>[2x]GAMNAQAEEFKKYLETNGIKPKQFHKKELIFNQWDPQEYCIFLYDGITKLTSISENGTIMNLQYYKGAFVIMSGFIDTETSVGYYNLEVISEQATAYVIKINELKELLSKNLTHFFYVFQTLQKQVSYSLAKFNDFSINGKLGSICGQLLILTYVYGKETPDGIKITLDNLTMQELGYSSGIAHSSAVSRIISKLKQEKVIVYKNSCFYVQNLDYLKRYGPKLDEWFYLACPATWGKLN

The major regulator of virulence factors in L. monocytogenes is the transcription activator PrfA, a member of the Crp/Fnr family of regulators. PrfAWT is a homodimer in which each monomer consists of an N-terminal domain (residues 1 to 108) and a C-terminal DNA-binding domain (residues 138 to 237) linked by a long α-helix (αC, residues 109 to 137). Two α-helices in the C-terminal domain, αE (residues 170 to 178) and αF (residues 183 to 197), constitute the two helices of the typical HTH motif present in many prokaryotic transcription factors. Glutathione binding stabilizes the DNA-binding helix-turn-helix (HTH) motif in a conformation compatible with DNA-binding, thereby allowing expression of PrfA-regulated virulence factors.

In addition, we found three new PrfA mutants in the remaining three strains—Leu to His substitution at residue 140 (PrfAL140H), Ala to Gly substitution at residue 218 (PrfAA218G), and Ala to Val substitution at residue 94 (PrfAA94V). All the previously identified PrfA* mutants, i.e., PrfAG145S, PrfAG145C, and PrfAL140F, could grow in this medium with G-6-P, as could the PrfA mutants PrfAL140H and PrfAA218G, whereas the strain carrying the PrfAA94V mutation was unable to grow. The PrfAG145S, PrfAG145C, and PrfAL140F mutants showed the highest expression levels, followed by PrfAA218G and PrfAL140H. To gain a deeper understanding of the PrfA* mutant proteins, the crystal structures of purified PrfAL140H, PrfAL140F, and PrfAA218G were determined as individual proteins and in complex with the PrfA hly promoter DNA. We expected that the crystal structures of PrfAL140H, PrfAL140F, and PrfAA218G would be similar to the PrfAG145S structure, since our in vivo characterization classified them as PrfA* mutations. However, their structures showed that each of the PrfA* variants had only one folded HTH motif, with the remaining structure residing in the PrfAWT conformation. The PrfAL140H, PrfAL140F, and PrfAA218G PrfA* mutants all had a folded HTH motif in one monomer of the homodimer but an uncollapsed central core structure. Consequently, we suggest that these mutant structures represent an intermediately activated form of the protein with features characteristic of both inactive and activated PrfA. The most striking structural difference between the inactive, intermediate-active, and fully active structures is the position of their recognition helices. When superimposed on monomer B, the recognition helix in monomer A is shifted up to 6 Å.>MTMVDREQLFKKALEIKFTQEWGENKATEVSTDITSKKAKYLRLGTAQSPRKR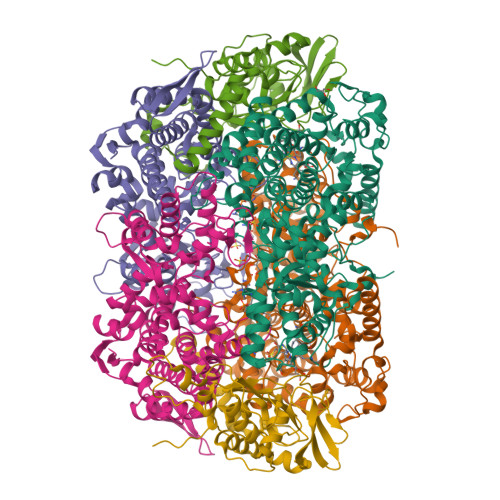EFEQYGKEIAAKRGLPGYDPKLHLGGIPLGQRQITPYVVSSTDTLCDGDDLHFVNNAAMQQMWDDIRRTVIVGMDLAHETLEKRLGKEVTPETINHYLEVLNHAMPGAAVVQEMMVETHPGLVDDCYVKVFTGDDELADEIDKRFLIDIDKQFGEEKAAQIKAAIGKTTWQAVHVPTIVVRTCDGATTSRWTAMQIGMSFIAAYRMCAGEAAVADLAYAAKHAALVGMGDMLPARRARGPNEPGGLQFGYLADIVQADRVTDDKVKASLEVVAAGAMLYDQIWLGSYMSGGVGFTQYATAAYTNNILDDFSYYGYEYAVDKYGGPAQAPATLETVKDIATETAIYAIEQYEYFPTLLEDQFGGSQRAAVVAAAAGIATGLATGNSQAGLSGWYLAQYLLKEAEGRLGFFGYDLQDQCGAANVFSYQSDEGLPLELRGPNYPNYAMNVGHQGEYAGIASSGHIGRGDAFVVNPLVKVAFADPLLNFDFTQVRKEFAKGAVREFDRCAGERALILPAK[4x];>MSDKVDIYSDRGKLLASDVDIMDLAPTRNRAIRTIIHDTKRTAAVNLGGIEKALANGRIGKVKKIPGKEMKLDIVANAERLAERVKELVQVNEGDDTTVEVLAGGKFLKVQVPSARLESGAEYVSSITASAAAITQAIIELFDVGIFDACMVKAAVWGDYPQTIGLNGGNVSSILEIPQKDEGLGFTLRNIMANHIAAITQRNAMNAAALSSILEQCGEFEMGNAIGMFERHQLLGLAYQGLNANNIVYETVKEQGKSGTIGTVVHSIVERALEDGVISVDKVAPSGYKFYKANDVMLWNAYAAAGSLAATMVNCGAARAAQCVSSTLLYFNDLLEKETGLPGCDYGKVQGTAVGFSFFSHSIYGGGGPGVFNGNHIVTRHSRGFAIPCVAAAVALDAGTQMFSPEMTSAVVGTVYGSIPEFREPIKTVAASL[4x];>[4x]MAYEPQYYPGNTSVAQNRRKHMSGNVEKLREISDEDLTAILGHRAPGSDYPSTHPPLAEMGEPDCPIREIVEPTPGAAAGDRIRYVQWTDSMYNAPATPYWRSYYAAINHRGVDPGTLSGRQIVEARERDVEVYGKMSIETEMTCPALAGLRGATVHGHSCRLQEDGVMFDMLDRRRLEGGTIIMDKDQVGVPLDRKVDLGKPMSEEEAAKRTTIYRVDNVPFRSDSEVVEWVQRIWELRTRYGFQPQ(7Z,19R,22R)-25-amino-22-hydroxy-16,22-dioxo-17,21,23-trioxa-22lambda~5~-phosphapentacos-7-en-19-yl (9Z)-octadec-9-enoate | C39 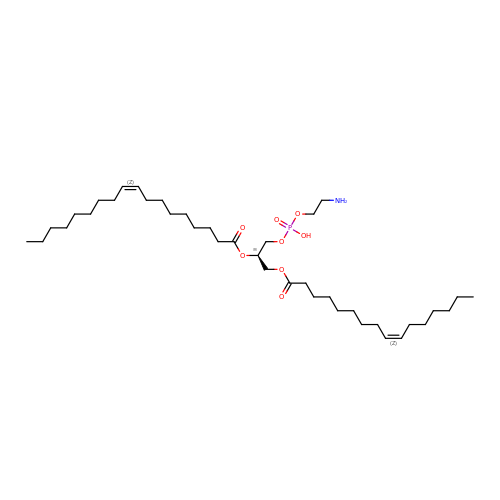H74 N O8 P | RAMNOXDFBNFSFC-AVWHJSSGSA-N> GHNTELLPIELDTLVGKGRFAEVYKAKLKQNTSEQFETVAVKIFPYEEYASWKTEKDIFSDINLKHENILQFLTAEERKTELGKQYWLITAFHAKGNLQEYLTRHVISWEDLRKLGSSLA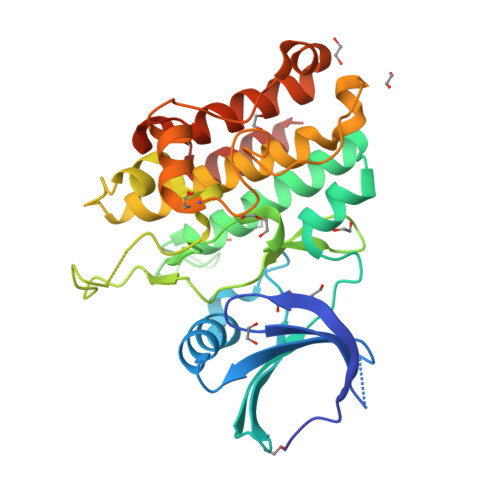RGIAHLHSDHTPCGRPKMPIVHRDLKSSNILVKNDLTCCLCDFGLSLRLDPTLSVDDLANSGQVGTARYMAPEVLASAMNLENVESFKQTDVYSMALVLWEMTSRCNAVGEVKDYEPPFGSKVREHPCVASMADNVLADAGRPEIPSFWLNHQGIQMVCETLTECWDHDPEARLTAQCVAERFSELEHLDRLSG6-bromanyl-8-oxidanyl-3~{H}-quinazolin-4-one | C8 H5 Br 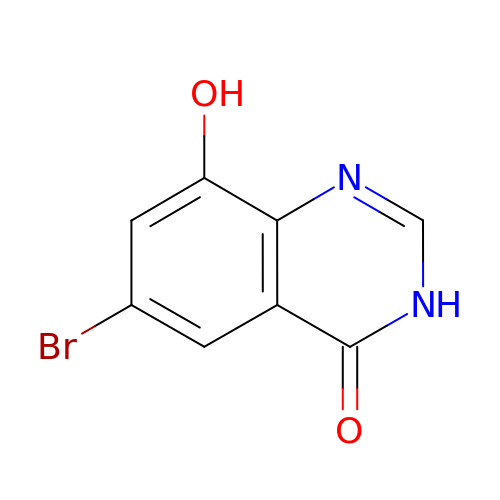N2 O2 | AUPAGWVOMYPVRN-UHFFFAOYSA-N> SPPKRLTREAMRNYLKERGDQTVLILHAKVAQKSYGNEKRFFCPPPCVYLMGSGWKKKKEQMERDGCSEQESQPCAFIGIGNSDQEMQQLNLEGKNYCTAKTLYISDSDKRKHFMLSVKMFYGNSDDIGVFLSKRIKVISKPSKKKQSLKNADLCIASGTKVALFNRLRSQTVSTRYLHVEGGNFHASSQQWGAFYIHLLDDDESEGEEFTVRDGYIHYGQTVKLVCSVTGMALPRLIIRKVDKQTALLDADDPVSQLHKCAFYLKDTERMYLCLSQERIIQFQATPCPKEQNKEMINDGASWTIISTDKAEYTFYEGMGPVLAPVTPVPVVESLQLNGGGDVAMLELTGQNFTPNLRVWFGDVEAETMYRCGESMLCVVPDISAFREGWRWVRQPVQVPVTLVRNDGVIYSTSLTFTYTPEP;> ARRKREHSTLWFPEGFSL

The Notch pathway relies on cell–cell contacts, where membrane-spanning Jagged and Delta-like ligands (DLLs) on signal-sending cells bind to Notch receptors on signal-receiving cells. This induces two sequential receptor cleavages, releasing the Notch intracellular domain (NICD), which translocates to the nucleus and forms a transcriptionally active complex with the Mastermind-like transcriptional coactivator and CSL (C promoter–binding factor 1, Suppressor of Hairless, Lag-1), also known as RBPJ (recombination signal–binding protein for immunoglobulin kappa J region). The ICDs of all four Notch receptor paralogs are composed of a CSL/RBPJ-associated molecule (RAM) domain, ankyrin repeats flanked by two nuclear localization sequences, a transactivation domain, and a C-terminal domain rich in proline, glutamic acid, serine, and threonine residues. The PIM target residue in Notch3 is in the RAM domain, which is required for canonical Notch signaling activity as it mediates binding with the DNA-binding protein CSL. Here, we demonstrate that PIM kinases phosphorylate Notch3 at a distinct site (serine 1673; corresponding to human NOTCH3 S1672) within the RAM domain, which is essential for binding to CSL.

To corroborate our predictive model, we crystallized mouse CSL (amino acid residues 53–474) in complex with the human N3RAM peptide (residues 1665–1682). These structural data also suggested that binding between N3RAM and CSL would be disrupted by phosphorylation at S1672. The binding site for S1672 resides in a small and hydrophobic cavity on CSL, suggesting that both the size and the negative charge on the phosphate group are likely to impair the binding of S1672 to CSL. In addition, the overall negative charge on the surface of CSL around the RAM-binding site is likely to repel the negative charge of the phosphorylated S1672. All these regions are conserved in N3ICD, except for the His–Gly motif, where the glycine residue is replaced by the PIM-targeted serine residue. To confirm this, we performed isothermal titration calorimetry (ITC) on mouse CSL with human RAM peptides, using either N3RAM, phosphorylated N3RAMpS1672, or N1RAM (residues 1754–1781), which was used as a positive binding control. Binding between naïve CSL and N3RAM was weaker (Kd = 0.187 μM) as compared with binding between CSL and N1RAM (Kd = 0.022 μM) and, in line with our predictive model, no binding could be detected between CSL and the phosphorylated N3RAMpS1672. In line with this observation, we were unable to produce crystal structures of the phosphorylated human N3RAMpS1672 peptide in complex with CSL (data not shown).>MSAAVAVPMDSTGPYRTVSHPENAPSGVDAGVGPSEWTHAYANPAHNAAFPVPDDAPEWIRNGVSWLFPEARAWPLANPPFGSKTYGAAEASVTQTQFYGNALGPSVVDGVVYAESDDMFAYAVNAKTGKLIWRASPVGNNLMGNPLVIGNTVYLSAGSVAFNFANVLRYAHNPSASARGLNVSFNGIYALNRSNGKLLWYFATPGETMATPAYDNNTLFIADGAGNAFGINATTGKQVWKTHVGGMDNMSSVTAYRHNIYFAMAIKPYLYCLNESN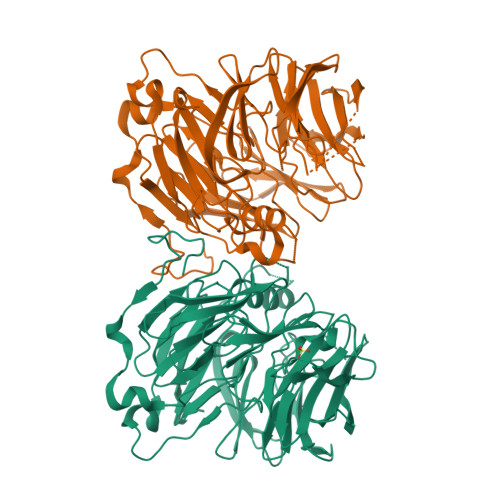GHIVWKGTIPGASNTGIGNVSPAAADGVVVLDATTKPQANKKAMFSNVIRAFDAKTGAVLWTRNMGSGGKIPAFKGGVPMIHNNIVYVGNPVASTYQAYELKTGKLLWTWHVPTKVAAGAGRSAPTYYKGLLYITTGQYIFVVNPATGKELHQHHIGGQFGIESPVIVGGTVYLTNSWDWIMAIPLKTISHGS[6x]> GSDASKLSSDYSLPDLINTRKVPNNWQTGEQASLE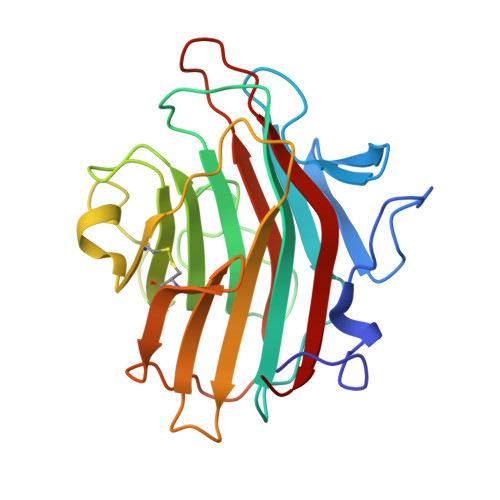EGRIVLTSNQNSKGSLWLKQGFDLKDSFTMEWTFRSVGYSGQTDGGISFWFVQDSNIPRDKQLYNGPVNYDGLQLLVDNNGPLGPTLRGQLNDGQKPVDKTKIYDQSFASCLMGYQDSSVPSTIRVTYDLEDDNLLKVQVDNKVCFQTRKVRFPSGSYRIGVTAQNGAVNNNAESFEIFKMQFFNGV>GGSPSAAIYNIDTSSESPDHYLVDHTLDGRVLFPATGYLSIVWKTLARALGLGVEQLPVVFEDVVLHQATILPKTGTVSLEVRLLEASRAFEVSENGNLVVSGKVYQWDDPDPRLFDHPESPTPNPTEPLFLAQAEVYKELRLRGYDYGPHFQGILEASLEGDSGRLLWKDNWVSFMDTMLQMSILGSAKHGLYLPTRVTAIHIDPATHRQKLYTLQDKAQVADVVVSRWLRVTVAGGVHISGLHTESAPRRQQEQQVPILEKFCFTPHTEEGCLSERAALQEELQLCKGLVQALQTKVTQQGLKMVVPGLDGAQIPRDPSQQELPRLLSAACRLQLNGNLQLELAQVLAQERPKLPEDPLLSGLLDSPALKACLDTAVENMPSLKMKVVEVLAGHGHLYSRIPGLLSPHPLLQLSYTATDRHPQALEAAQAELQQHDVAQGQWDPADPAPSALGSADLLVCNCAVAALGDPASALSNMVAALREGGFLLLHTLLRGHPLGDIVAFLTSTEPQYGQGILSQDAWESLFSRVSLRLVGLKKSFYGSTLFLCRRPTPQDSPIFLPVDDTSFRWVESLKGILADEDSSRPVWLKAINCATSGVVGLVNCLRREPGGNRLRCVLLSNLSSTSHVPEVDPGSAELQKVLQGDLVMNVYRDGAWGAFRHFLLEEDKPEEPTAHAFVSTLTRGDLSSIRWVCSSLRHAQPTCPGAQLCTVYYASLNFRDIMLATGKLSPDAIPGKWTSQDSLLGMEFSGRDASGKRVMGLVPAKGLATSVLLSPDFLWDVPSNWTLEEAASVPVVYSTAYYALVVRGRVRPGETLLIHSGSGGVGQAAIAIALSLGCRVFTTVGSAEKRAYLQARFPQLDSTSFANSRDTSFEQHVLWHTGGKGVDLVLNSLAEEKLQASVRCLATHGRFLEIGKFDLSQNHPLGMAIFLKNVTFHGVLLDAFFNESSADWREVWALVQAGIRDGVVRPLKCTVFHGAQVEDAFRYMAQGKHIGKVVVQVLAEEPEAVLKGAKPKLMSAISKTFCPAHKSYIIAGGLGGFGLELAQWLIQRGVQKLVLTSRSGIRTGYQAKQVRRWRRQGVQVQVSTSNISSLEGARGLIAEAAQLGPVGGVFNLAVVLRDGLLENQTPEFFQDVCKPKYSGTLNLDRVTREACPELDYFVVFSSVSCGRGNAGQSNYGFANSAMERICEKRRHEGLPGLAVQWGAIGDVGILVETMSTNDTIVSGTLPQRMASCLEVLDLFLNQPHMVLSSFVLAEKAAAYRDRDSQRDLVEAVAHILGIRDLAAVNLDSSLADLGLDSLMSVEVRQTLERELNLVLSVREVRQLTLRKLQELSSKADEASELACPTPKEDGLAQQQTQLNLRSLLVNPEGPTLMRLNSVQSSERPLFLVHPIEGSTTVFHSLASRLSIPTYGLQCTRAAPLDSIHSLAAYYIDCIRQVQPEGPYRVAGYSYGACVAFEMCSQLQAQQSPAPTHNSLFLFDGSPTYVLAYTQSYRAKLTPGCEAEAETEAICFFVQQFTDMEHNRVLEALLPLKGLEERVAAAVDLIIKSHQGLDRQELSFAARSFYYKLRAAEQYTPKAKYHGNVMLLRAKTGGAYGEDLGADYNLSQVCDGKVSVHVIEGDHRTLLEGSGLESIISIIHSSLAEPRVSVREGLESRGPHHHHHH[2x]

Fatty acid synthase (FASN) catalyzes the de novo synthesis of palmitate, a 16-carbon chain fatty acid that is the primary precursor of lipid metabolism and an important intracellular signaling molecule. In contrast, Type I FAS found in eukaryotes and some actinobacteria are large complexes of multi-domain protomers that are composed of one or two repeating polypeptides that are each encoded by a single gene and organized in a symmetric or pseudo-symmetric assembly. In humans, the FASN gene encodes a 273 kDa polypeptide that comprises the catalytic domains necessary for palmitate synthesis, which further homodimerizes into a pseudo-symmetric complex. The contact point of the condensing and modifying regions is the neck region, a flexible linker composed of two short unstructured loops which allow for continuous swinging and swiveling motions of the two regions relative to each other, maximizing ACP accessibility to all catalytic centers. hFASN is a validated anti-cancer target and is over-expressed in solid tumors including those from breast, prostate, liver, and lung tissues.

The engineered protein enables electron cryo-microscopy (cryoEM) structure determination of the core modifying region of hFASN to 2.7 Å resolution. The isolated modifying region of hFASN produced via the TEV cleavage method demonstrated adequate orientation distribution to enable 3-dimensional reconstruction of a cryoEM map of the complex into which an atomic model for the core modifying region was built. CryoEM analysis of the modifying region revealed an arch shaped homodimer composed of two of each of the DH, ΨME, ΨKR, ER, and KR domains while lacking density for the C-terminal ACP & TE domains. No cryoEM densities were observed in the 3D reconstruction that could be assigned to the ACP and TE domains, consistent with the inherent flexibility of these domains relative to the core. Many residues within the ΨME and ΨKR domains lacked defined side chain densities, although backbone density was clearly defined. This observation suggested the presence of significant conformational dynamics within the two pseudo domains at the periphery of the hFASN core modifying region. Our structure of the human core modifying region aligns well with that of porcine FASN (78% sequence identity) with a backbone RMSD of 1 Å, indicating its structural integrity in isolation. Surprisingly, close examination of the human DH domain revealed a close-ended catalytic cavity as opposed to the porcine homolog where DH domain has an open-ended cavity. This is due to the presence of a leucine residue (i.e., L1097) instead of an alanine at the back end of the catalytic cavity in the human protein.>GPDLVQKLKVLRHELSLQQPQAGHCRIEVSREEIFEESYRQIMKMRPKDLKKRLMVKFRGEEGLDYGGVAREWLYLLCHEMLNPYYGLFQYSTDNIYMLQINPDSSINPDHLSYFHFVGRIMGLAVFHGHYINGGFTVPFYKQLLGKPIQLSDLESVDPELHKSLVWILENDITPVLDHTFCVEHNAFGRILQHELKPNGRNVPVTEENKKEYVRLYVNWRFMRGIEAQFLALQKGFNELIPQHLLKPFDQKELELIIGGLDKIDLNDWKSNTRLKHCVADSNIVRWFWQAVETFDEERRARLLQFVTGSTRVPLQGFKALQGSTGAAGPRLFTIHLIDANTDNLPKAHTCFNRIDIPPYESYEKLYEKLLTAVEET[4x]

The structure of SMURF1 is typical of a NEDD4 subfamily member, with a N-terminal C2 domain for cellular membrane localization, WW domains for target recognition, and a catalytic HECT domain that binds E2 and mediates target ubiquitylation through a surface-protruding catalytic cysteine. At the cellular level, SMURF1 acts as a negative regulator of bone morphogenetic protein (BMP) signaling, which modulates cell migration, proliferation, and apoptosis. Ubiquitin transfer requires a motion facilitated by a flexible hinge that connects the HECT domain N- and C-lobes. To gain structural insights into the mechanism of selective inhibition, we crystallized the HECT domains of both SMURF1 and SMURF2, without and with a representative SMURF1 inhibitor, compound-8 (Cpd-8), and determined structures at 2.05–2.75 Å resolution.

In the absence of the inhibitor, the HECT domains of SMURF1 and SMURF2 adopted a highly similar architecture, comprising N- and C-lobes connected by a flexible glycine-containing hinge (residues G634–D639). Across all 28 HECT domain structures (including SMURF1), the α helix10 (αH10) comprises two and a half turns and ends with the conserved glycine, which provides flexibility between the N- and C-lobes through its high tolerance of ϕ/Ψ dihedral angles. To determine amino acid sequences critical for SMURF1 activity, we employed a fast Fourier transformation-based multiple alignment. These analyses demonstrated that G634, which stems the SMURF1 hinge, is invariant in all HECT sequences across animal, plant, and fungal kingdoms and in all 28 HECT domain structures. Function of the hinge is facilitated by its length and the flexibility provided by amino acid residues with a tolerance to a wide range of ϕ/Ψ dihedral angles. (A) In unbound-SMURF1, I631 of the αH10 (and other nearby residues) occupies the cryptic cavity, which is therefore not available for small molecule inhibitor binding.>[2x]MTKSSKDICSENEGKKNGKSGFFSTSFKYVLSACIASFIFGYQVSVLNTIKNFIVVEFEWCKGEKDRLNCSNNTIQSSFLLASVFIGAVLGCGFSGYLVQFGRRLSLLIIYNFFFLVSILTSITHHFHTILFARLLSGFGIGLVTVSVPMYISEMTHKDKKGAYGVMHQLFITFGIFVAVMLGLAMGEGPKADSTEPLTSFAKLWWRLMFLFPSVISLIGILALVVFFKEETPYFLFEKGRIEE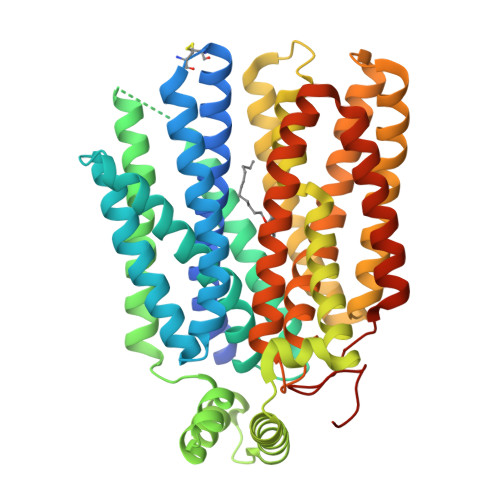SKNILKKIYETDNVDEPLNAIKEAVEQNESAKKNSLSLLSALKIPSYRYVIILGCLLSGLQQFTGINVLVSNSNELYKEFLDSHLITILSVVMTAVNFLMTFPAIYIVEKLGRKTLLLWGCVGVLVAYLPTAIANEINRNSNFVKILSIVATFVMIISFAVSYGPVLWIYLHEMFPSEIKDSAASLASLVNWVCAIIVVFPSDIIIKKSPSILFIVFSVMSILTFFFIFFFIKETKGGEIGTSPYITMEERQKHMTKSVV> XXXXXXXXXXXXXXXXXXXXXXXXXXXXXXXXXXXXXXXXXXXXXXXXXXLPWWAVGASLIAANISAEQ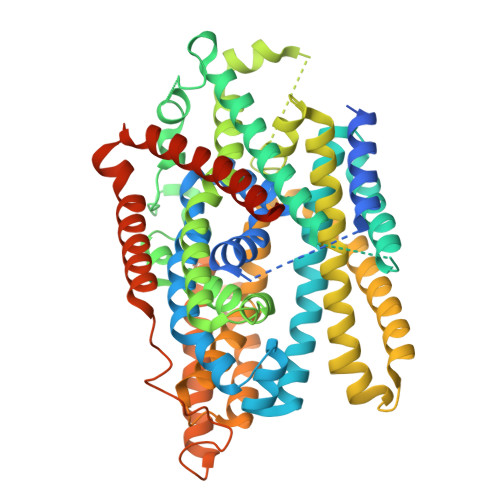FIGMSGSGYSIGLAIASYEWMSAITLIIVGKYFLPIFIEKGIYTIPEFVEKRFNKKLKTILAVFWISLYIFVNLTSVLYLGGLALETILGIPLMYSILGLALFALVYSIYGGLSAVVWTDVIQVFFLVLGGFMTTYMAVSFIGGTDGWFAGVSKMVDAAPGHFEMILDQSNPQYMNLPGIAVLIGGLWVANLYYWGFNQYIIQRTLAAKSVSEAQKGIVFAAFLALIVPFLVVLPGIAAYVITSDPQLMASLGDIAATNLPSAANADKAYPWLTQFLPVGVKGVVFAALAAAIVSSLASMLNSTATIFTMDIYKEYISPDSGDHKLVNVGRTAAVVALIIAALIAPMLGGIGQCFQYIQEYTGLVSPGILAVFLLGLFWKKTTSKGAIIGVVASIPFALFLKFMPLSMPFMDQMLYTLLFTMVVIAFTSLSTSINDDDPKGISVTSSMFVTDRSFNIAAYGIMIVLAVLYTLFWVNADAEITLIIFGVMAGVIGTILLISYGIKKLIKASYKSGGSPGHHHHHH> MIERLNSPFLRAAALFTIVAFSSLISTAALAENNPSDTAKKFKVVTTFTIIQDIAQNIAGDVAVVESITKPGAEIHDYQPTPRDIVKAQSADLILWNGMNLERWFEKFFESIKDVPSAVVTAGITPLPIREGPYSGIANPHAWMSPSNALIYIENIRKA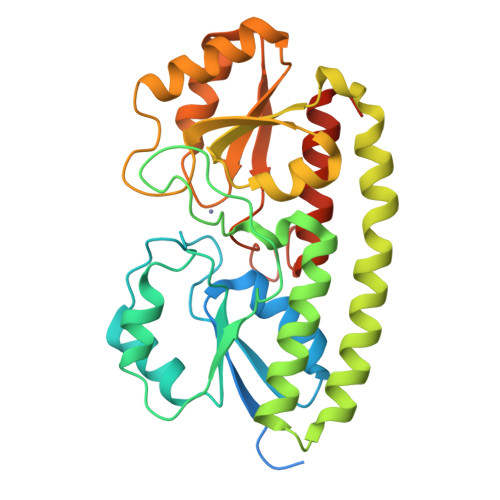LVEHDPAHAETYNRNAQAYAEKIKALDAPLRERLSRIPAEQRWLVTSEGAFSYLAKDYGFKEVYLWPINAEQQGIPQQVRHVIDIIRENKIPVVFSESTISDKPAKQVSKETGAQYGGVLYVDSLSGEKGPVPTYISLINMTVDTIAKGFGQLEHHHHHHHHHH>GSSTNYGTIKWIFHALVFSYISFALISDKRYQKKEPL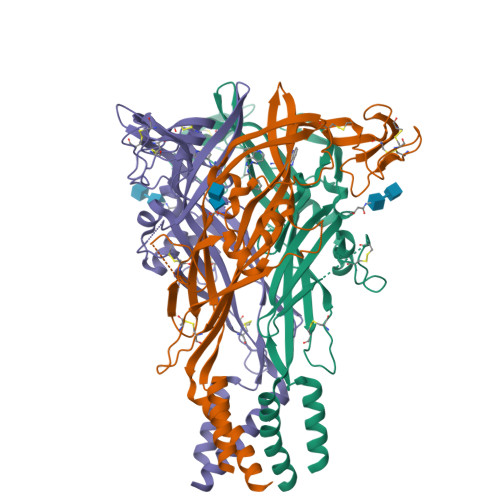ISSVHTKVKGIAEVKAEILENGMKKMVSGVFDTADYTFPLQGNSFFVMTNFIKTEGQQQGLCPDFPTARTICSSDRGCKKGRMDPQSKGIQTGRCVVYKERLKTCEVSAWCPIEEVKDAPRPALLNSAENFTVLIKNNIDFPGHNYTTRNILPGVNITCTFHKTQNPQCPIFRLGDIFQETGDSFSDVAIQGGIMGIEIYWDCNLDGWFHHCRPKYSFRRLDDKTTSESLYPGYNFRYAKYYKENNVEKRTLIKVFGIRFDILVFGTGGKFNVIQLAVYIGSVISYFGLATVFIDILINTYSASS[2x]> GPLGS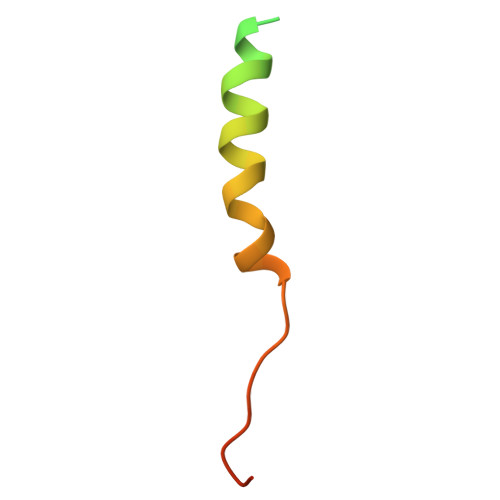MAAAEEGASVGAEADRELEELLESALDDFDKAKPSPAPPSTTTA> ASEKVEMNLVTSQGVGQSIGSVTITETDKGLEFSPDLKALPPGEHGFH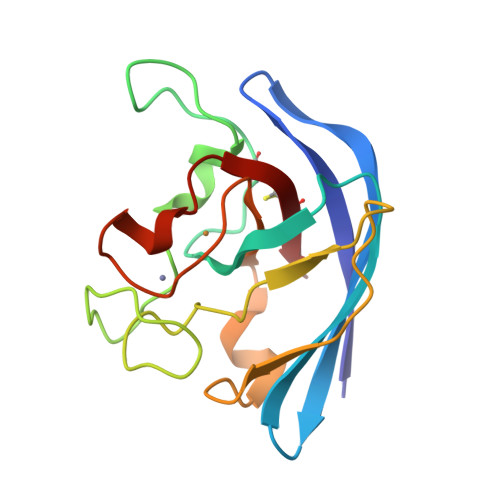IHAKGSCQPATKDGKASAAESAGGHLDPQNTGKHEGPEGAGHLGDLPALVVNNDGKATDAVIAPRLKSLDEIKDKALMVHVGGDNMSDQPKPLGGGGERYACGVIK>[2x]MNNMNVIIADDHPIVLFGIRKSLEQIEWVNVVGEFEDSTALINNLPKLDAHVLITDLSMPGDKYGDGITLIKYIKRHFPSLSIIVLTMNNNPAILSAVLDLDIEGIV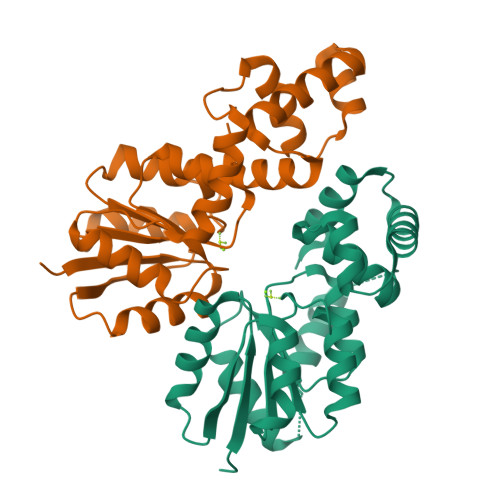LKQGAPTDLPKALAALQKGKKFTPESVSRLLEKISAGGYGDKRLSPKESEVLRLFAEGFLVTEIAKKLNRSIKTISSQKKSAMMKLGVENDIALLNYLSSVTLSPTDKE4-(4-fluorophenyl)-1H-imidazole 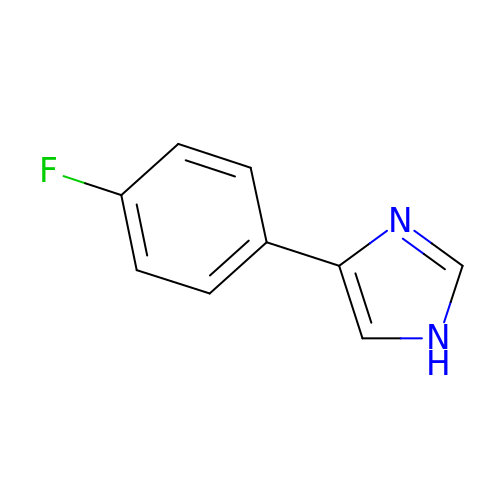| C9 H7 F N2 | QYDAFWKRBZYBOB-UHFFFAOYSA-N>[2x]MNVTVDQSTLAGATRGIVRGGETLKEHRDRLMAATKATGRYAGLKTLELREREPILYNKLFSRLRAGVVDARETAKKIAASPIVEQEGELCFTLYNAAGDSLLTSTGIIIHVGTMGAAIKYMIENNWEANPGVHDKDIFCNNDSLIGNVHPCDIHTIVPIFWEGELIGWVGGVTHVIDTGAVGPGSMATGQVQRFGDGYSITCRKVGANDTLFRDWLHESQRMVRTTRYWMLDERTRIAGCHMIRKLVEEVVAEEGIEAYWKFAYEAVEHGRLGLQARIKAMTIPGTYRQVGFVDVPYAHEDVRVPSDFAKLDTIMHAPCEMTIRRDGTWRLDFEGSSRWGWHTYNAHQVSFTSGIWVMMTQTLIPSEMINDGAAYGTEFRLPKGTWMNPDDRRVAFSYSWHFLVSAWTALWRGLSRSYFGRGYLEEVNAGNANTSNWLQGGGFNQYDEIHAVNSFECAANGTGATAVQDGLSHAAAIWNPEGDMGDMEIWELAEPLVYLGRQIKASSGGSGKYRGGCGFESLRMVWNAKDWTMFFMGNGHISSDWGLMGGYPAASGYRFAAHKTNLKELIASGAEIPLGGDTDPENPTWDAMLPDAQIKRDKQAITTEEMFSDYDLYLNYMRGGPGFGDPLDREPQAVADDINGGYVLERFAGEVYGVVVRKGADGQYGVDEAGTAAARAQIRKDRLAKSVPVSEWMKGEREKILAKDAGTQVRQMFAASFKLGPRFEKDFRTFWSLPDSWTLPEEEIGVPTYGSRYSMDISELPDVHTVQFVEE;>MHHHHHHSSGMNVPVGHLRNVQVLGIDAGGTMTDTFFVD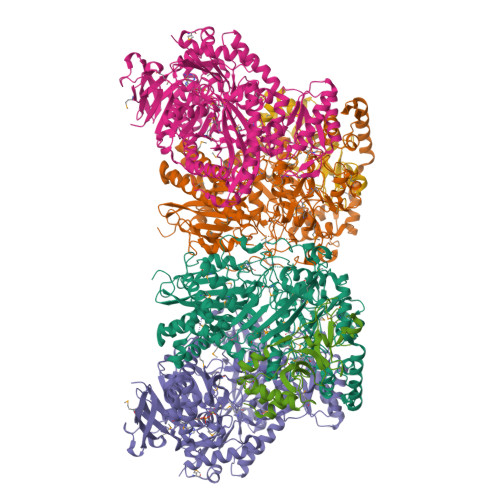QDGDFVVGKAQSTPQNEALGLIASSEDGLANWGMSLHEALAQLQTGVYSGTAMLNRVVQRKGLKCGLIVNRGMEDFHRMGRAVQSHLGYAYEDRIHLNTHRYDPPLVPRHLTRGVVERTDMIGTQVIPLREDTARDAARDLIAADAEGIVISLLHSYKNPENERRVRDIVLEEVEKSGKKIPVFASADYYPVRKETHRTNTTILEGYAAEPSRQTLSKISNAFKERGTKFDFRVMATHGGTISWKAKELARTIVSGPIGGVIGAKYLGEVLGYKNIACSDIGGTSFDVALITQGEMTIKNDPDMARLVLSLPLVAMDSVGAGAGSFIRLDPYTRAIKLGPDSAGYRVGVCWKESGIETVTISDCHMVLGYLNPDNFLGGAVKLDRQRSVDAIKAQIADPLGLSVEDAAAGVIELLDSDLRDYLRSMISGKGYSPASFVCFSYGGAGPVHTYGYTEGLGFEDVIVPAWAAGFSAFGCAAADFEYRYDKSLDINMPTETPDTDKEKAAATLQAAWEELTKNVLEEFKLNGYSADQVTLQPGYRMQYRGQLNDLEIESPLAQAHTAADWDQLTDAFNATYGRVYAASARSPELGYSVTGAIMRGMVPIPKPKIPKEPEEGETPPESAKIGTRKFYRKKRWVDAQLYHMESLRPGNRVMGPAVIESDATTFVVPDGFETWLDGHRLFHLREV[2x];>MAYTRSKIVDLVDGKIDPDTLHQMLSTPKDPERFVTYVEILQERMPWDDKIILPLGPKLFIVQQKVSKKWTVRCECGHDFCDWKDNWKLSARVHVRDTPQKMEEIYPRLMAPTPSWQVIREYFCPECGTLHDVEAPTPWYPVIHDFSPDIEGFYQEWLGLPVPERADA[2x]> MISDSMTVEEIRLHLGLALKEKDFVVDKTGVKTIEIIGASFVADEPFIFGALNDEYIQRELEWYKSKSLFVKDIPGETPKIWQQVASSKGEINSNYGWAIWSEDNYAQYDMCLAELGQNPDSRRGIMIYTRPSMQFDYNKDGMSDFMSTNTVQYLIRDKKINAVVNMRSNDVVFGFRNNYAWQKYVLDKLVSDLNAGDSTRQYKAGSIIWNVGSLHVYSRHFYLVDHWWKTGET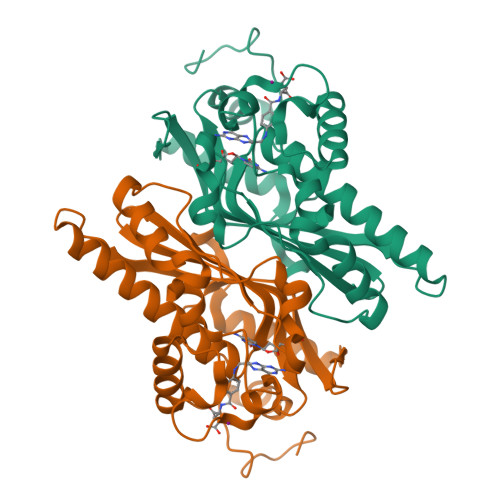HISKKDYVGKYA> ELCDDDPPEIPHATFKAMAYKEGTMLNCECKRGFRRI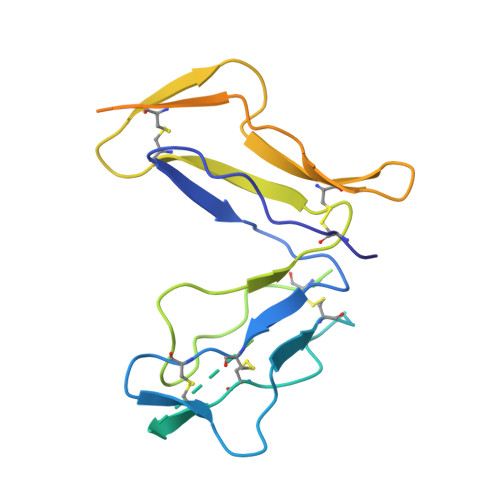KSGSLYMLCTGNSSHSSWDNQCQCTSSATRQTTKQVTPQPEEQKERKTTEMQSPMQPVDQASLPGHCREPPPWENEATERIYHFVVGQMVYYQCVQGYRALHRGPAESVCKMTHGKTRWTQPQLICTGEMETSQFPGEEKPQASPEGRPESETSCLVTTTDFQIQTEMAATMETSIFTTE>[2x]MDHLPIFCQLRDRDCLIVGGGDVAERKARLLLEAGARLTVNALTFIPQFTVWANEGMLTLVEGPFDETLLDSCWLAIAATDDDTVNQRVSDAAESRRIFCNVVDAPKAASFIMPSIIDRSPLMVAVSA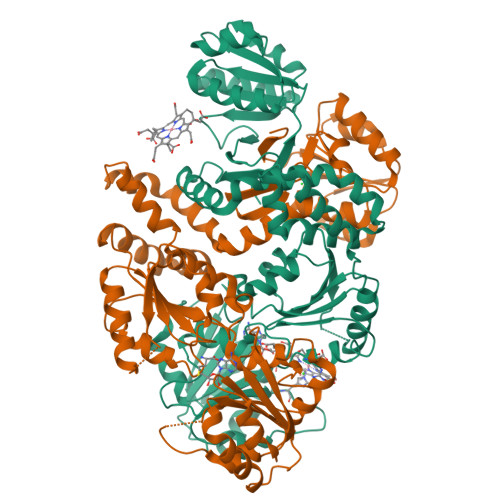GGTSPVLARLLREKLESLLPQHLGQVARYAGQLRARVKKQFATMGERRRFWEKFFVNDRLAQSLANADEKAVNATTERLFSEPLDHRGEVVLVGAGPGDAGLLTLKGLQQIQQADIVVYDRLVSDDIMNLVRRDADRVFVGKRAGYHCVPQEEINQILLREAQKGKRVVRLKGGDPFIFGRGGEELETLCHAGIPFSVVPGITAASGCSAYSGIPLTHRDYAQSVRLVTGHLKTGGELDWENLAAEKQTLVFYMGLNQAATIQEKLIAFGMQADMPVALVENGTSVKQRVVHGVLTQLGELAQQVESPALIIVGRVVALRDKLNWFSNH1-benzyl-2-(4-{[(2R)-2-(2-phenyl-1H-benzimidazol-1-yl)pent-4-en-1-yl]oxy}phenyl)-1H-benzimidazole | C38 H32 N4 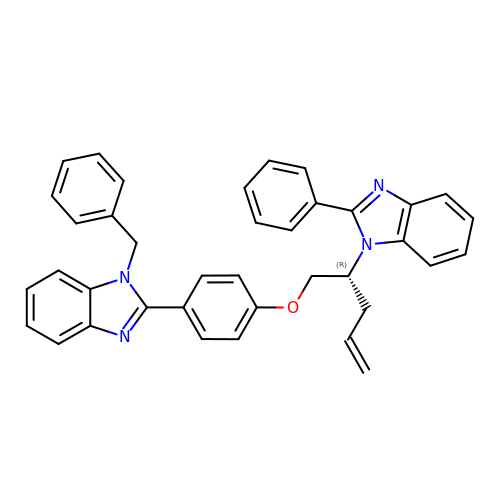O | VETKHSOXOHNPCG-WJOKGBTCSA-N>[3x]MVRNNNRRRQRTQRIVTTTTQTAPVPQQNVPKQPRRRRNRARRNRRQGRAMNMGALTRLSQPGLAFL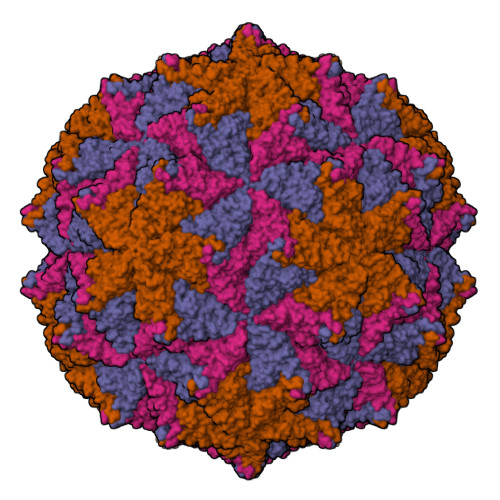KCAFAPPDFNTDPGKGIPDRFEGKVVTRKDVLNQSINFTANRDTFILIAPTPGVAYWVADVPAGTFPISTTTFNAVNFPGFNSMFGNAAASRSDQVSSFRYASMNVGIYPTSNLMQFAGSITVWKCPVKLSNVQFPVATTPATSALVHTLVGLDGVLAVGPDNFSESFIKGVFSQSVCNEPDFEFSDILEGIQTLPPANVTVATSGQPFNLAAGAEAVSGIVGWGNMDTIVIRVSAPTGAVNSAILKTWACLEYRPNPNAMLYQFGHDSPPCDEVALQEYRTVARSLPVAVIAAQN;>ASMWERVKSIIKSSLAMASNVPGPIGIAASGLSGLSALFEGFGF[3x]>[2x]MSRQASRLDAKKVNSEFLTLTYGALVTQMLRDFENAEDVNKQLERIGYNMGMRLIEDFLARTSAPRCLEMRETADRIQQAFRIYLNIQPTISNWSPASDEFSLVFDSNPLTEFVELPPDLTNLRYSAILSGCIRGALEMVQLEVQCWFVQDQLKGDNVTELRVKFVRRLEEVIPAGED;> MSEEILFDCLHAEIVNYCLDSNKEHDLATLEYIGFTTGYRLIERLTREVSRFKDELETMKFICTD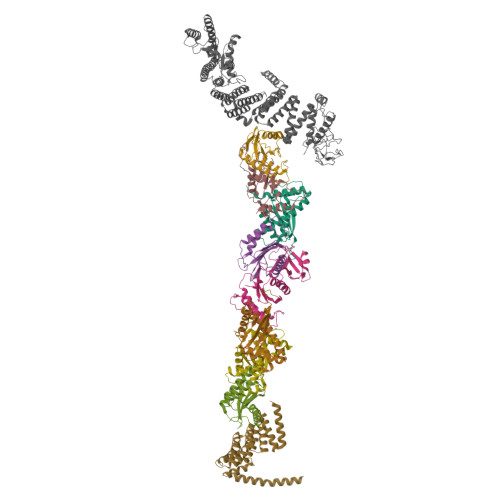FWMLIYKKQVDNLRTNNHGMYVVQDKAFRFLTRISPGTKQLEHAPKFVAFTCGLVRGALSNLGINSTVTAEVQSIPACKFHIEVNRN;> MTIFNLYIFDKFGTLLHYAEWNRTKKSGITREEEAKLTYGMLFSIKSFVSKISPHDPKEGFLYYKTNRYALHYLETPSGLKFVLNTDTTAINVKELLQQLYAKVWVEFVVRDPLWTPGTVVTSELFQSKLDEFVRQSPIFGIRNI;> MIIYGVYIVSKSGGLIFNLDNNVPRIEHEKTFTYPLDLVLDYDSKKVSVSFNRKDGINVGHVLVAVNGMPVNGVTLDDGRDVRTTLDAPENYPINLKFSRPKMTTNEKIFLASMFYPLFAIASQLSPEPKSSGIEILEADTFTLHCFQTLTGIKFIIISETGLNGIDLLLRKVYELYSDYVLKNPFYSLEMPIRCELFDNKLQELLAQVEKTGISNIDK;> MSTYYFVIVGQNDNPIYEKEFSTVNKELRKEDHRHLTQFIAHAALDLVDEHKWKTANMQLKSIDRFNQWFVSAFITASQIRFIIVHDNKNDEGIKNFFNEMYDTYIKNSMNAFYRINTPIKSPMFEKKSEIFGRKYLLS;> MEKLEALKISSMRPRSNILDRPLSKGKTEVSQSIVALLFSEIVQYSQSRVFTVPELQTRLHDLGQDVGTRIIDLYFVRERSSKRETKLTQMLLFVKTTVWKNLFGKEAEKLEHANDDERTYYIIEKEPLVNTFISVPKDKGSLNCANFTAGIVEAVLTNCGFPCKVTAHWHKGTTYMVKFEDFVIARDKQMEEK;> MAFCIAVIGKDNAPLYLTTSDMEQELELQYHVNAALDVVEEKCLIGKGAPESKELYLGLLYSTENHKIYGFVTNTRVKFIVVIDSSNVALRENEVRAIFRNLHLLYTDAICNPFYIPGESLTSKKFDRAVQKLMSGTA;> DNLRHFVQDYAVRALIPYIEHLVAILAEGVTNKKGVSKSLLSATKRWFVTSKPGAGANNQNAVIYTNESAELQTRKLGDLYFMFGHYNLAFQSYHQAKRDFNADSAWQYYAGALEMAALSAFMLGTAQRKTYDYMEDAIVCYLTVCKLQQFATRATLLSMECLKTARLYSEVAKQLIRMTNEESDLRSALLLEQAAYCFLVTQPPMHRKYAFHIVLAGNRYSRAGQRKHAYRCYRQAYQVFQKREW;> MTMDATALPSELLVTPQPLVGFCGLDTARVSVHKAVWEAFSGSLQRKAADRAAVQYKLLPPNYEFPVAKPKRASYEWYHPKGILKRNWMLKHLHVLPSVVVLFQDMEWNDLQWTEKQVQCAAIVQALKNTLQERNTRLCLVLLQRAAPLPPGEDLLAAERAASLTNACGITSKMLFILPHTEHLTGYALRLESAFLDMAQSYYALMSKRIRNHRDQLTAAHTSLKIRHQFKLGFVAEMRQDFSTGQKHYFQAYANLDEIRINDGNCLEIKTLAGFLNYKICRLMFKLKTPRDAINQFIIHVEKHKSRVGFKDLAFEHHAWLSTQHSVFAELFCEAIKNGLPALQTQHPGIYYHKAAEFVMKRRDAAMEAYAAMQASSEATPTPIQNPLSLYTEFFGIRAVKTGDLVAEQQANMQLCDQERSYNHSAAIIALLSQAMAQFKIYKCLRFRKKLAIDMAEEYLKSGDHAKALTLYSLMLPDYRQEKWTTIFTDVLLKTLRCALLSGSVADYIACSVEALSLRHQSDQSERILILENLWQVFQGVPPMPKTQLTPEAQALWTSALANVKSPIQIDLDKVNDVVEMCATFERVQLSNDDLLQLQLIVRVLTDIPLRIRSFHVILADAGNPQNSYKLEALKYFCFPTLTQLRGQKQPDDEQLENPSQEPKNFEKNMRLEPGSYYQLFCSTEAQQFHENTQLRIVRLEAHMGTDQVAALLTCSSN> 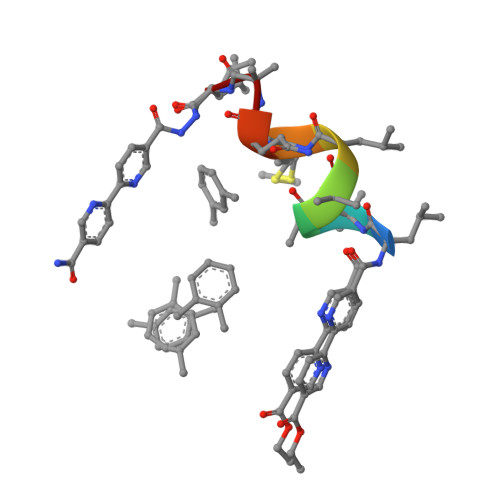LAAALMQAL The precursor PdDfsB is cleaved by subtilisin to yield biologically active Slf, and the chemical gradients of both proteins between two growing colonies could be accurately modelled. However, remarkably, the dfsB gene is widely distributed across Gram-positive and to some extent Gram-negative bacterial kingdoms (PFAM entry DUF1706). PdDfsB adopts a four-helical bundle core structure that belongs to the DinB structural superfamily. The most strongly conserved region of PdDfsB is the C-terminal helix, which is present within the mature Slf sequence.

There is even a homologue (irc4) within the yeast genome. The first of these two contain many homologues from Gram-positive bacteria, including pathogenic species, and also the yeast DfsB homologue, IRC4. This protein from S. cerevisiae is most closely related to the Lactobacillus DfsB homologue, implying a long history of association between these disparate organisms. An intriguing question is whether yeast secretes a processed form of IRC4, analogous to Slf, which goes on to control the population of co-cultured Lactobacillus species. We were able to express, purify and obtain crystal structures for DfsB homologues from Clostridium difficile 630 and Escherichia coli UTI89, as well as of IRC4 from S. cerevisiae. The overall structures of CdDfsB, EcDfsB and IRC4 are identical with that of PdDfsB, with strong conservation of overall topology and surface charge, particularly in the C-terminal helix.

>MRGSHHHHHHGSMREYTSKKELKEEIEKKYEKYDAEFETISESQKDEKVETVDRTPSENLSYQLGWVNLLLEWEAKEIAGYNVETPAPGYKWNNLGGLYQSFYKKYGIYSIKEQRAKLREAVNEVYKWISTLSDDELFQAGNRKWATTKAMWPVYKWIHINTVAPFTNFRGKIRKWKRLVPEEQRIKRRKI[2x]Listeria monocytogenes is a well-characterized food-borne pathogen capable of placental crossing and is thus ideal for probing this barrier. Pathogenic L. monocytogenes strains contain genes for 25 known members of this protein family, which share a common overall structure that includes a secretory signal sequence at the N-terminus and a large leucine-rich repeat (LRR) domain, a motif frequently implicated in protein-protein interactions. The two best-characterized internalins, InlA and InlB, contribute to L. monocytogenes invasion of epithelial cells and hepatocytes by binding to their cognate host cell surface receptors, E-cadherin and c-Met respectively.

Using pregnant guinea pigs, which have a placental structure that closely resembles humans, we identified a protein (InlP) secreted by the bacterial pathogen Listeria monocytogenes that strongly promotes placental infection. Recently, we used an unbiased genetic screen in a pregnant guinea pig model of listeriosis to identify L. monocytogenes genes that contribute specifically to infection of the placenta.. One gene identified in this screen encodes InlP, a member of the internalin family of proteins. While most internalins are predicted to be anchored to the bacterial cell surface via attachment to the peptidoglycan cell wall or to lipoteichoic acids, four of them, including InlP, lack obvious anchoring domains and are predicted to be secreted by the bacterium. Here, we solved the crystal structure of InlP, and identified Afadin, a cytoplasmic protein that localizes to adherens junctions as a binding partner of InlP. In this work, we identify the host cell cytoplasmic protein afadin as a major binding partner for InlP, and demonstrate that the InlP-afadin interaction specifically enhances L. monocytogenes transcytosis—that is, the ability of L. monocytogenes to exit from the basal face of an infected polarized epithelial monolayer, consistent with its potential contribution to placental infection. We demonstrate that InlP decreases the magnitude of traction stresses epithelial cells exert on an underlying extracellular matrix, and furthermore, that InlP facilitates bacterial spread from infected epithelial monolayers into an underlying compartment. In human placental organ cultures bacteria deficient in InlP were impaired in their ability to spread from infected placental cytotrophoblasts into the underlying fetal stroma.

> SNAASDLYPLPAPIIDVFPDDGLAKDMAKNLNKDSVNDVIDQDDLDALTGLGFETSTITNDSMQLLERAMFNNVTDVSIMEFGAKLTEFPDITTIPHLKTLFFADPPGRLTRNLSLPNYQNYPEMDTITMSGNNLIGSIPDFTGMPALKQLYMSEMLITSDELPNFNNIPLLITLDLSSNQLTTIPDFQNIPNLTFLDLNANLLTNTPDFQNLPKLTDLNLRHNNLTGTMVNYTNLPSLESLNLDYNFLTELPSNVLDTIYVQSQNGELPDQTINQGDTCTIDLPIYFQMEETNMLVSPEVTGEYIGISVIQLPTTVNEEGNTITVDTSALSPGEYKLDVSYNHNYATGGVCSYDWNVTIN>MTDRDRLRPPLDERSLRDQLIGAGSGWRQLDVVAQTGSTNADLLARAASGADIDGVVLIAEHQTAGRGRHGRGWAATARAQIILSVGVRVVDVPVQAWGWLSLAAGLAVLDSVAPLIAVPPAETGLKWPNDVLARGGKLAGILAEVAQPFVVLGVGLNVTQAPEEVDPDATSLLDLGVAAPDRNRIASRLLRELEARIIQWRNANPQLAADYRARSLTIGSRVRVELPGGQDVVGIARDIDDQGRLCLDVGGRTVVVSAGDVVHLR[2x]

Acetyl Coenzyme A Carboxylase (ACC), an important enzyme that catalyzes the first reaction of fatty acid biosynthesis, is biotinylated by biotin acetyl-CoA carboxylase ligase (BirA). The Mtb-BirA molecule is composed of two domains; N-terminal domain 1 comprises of 7 β-strands (β1: 29–32, β2: 55–59, β3: 82–88, β4: 124–126, β5: 131–133, β6: 137–147 and β7: 150–158) and 6 α-helices (α1: 13–20, α2: 39–48, α3: 95–114, α4: 173–176, α5: 183–203, α6: 206–215), while C-terminal domain 2 is a SH3 domain with 5 strands forming an antiparallel β-sheet (β8: 220–227, β9: 231–240, β10: 246–250, β11: 253–257 and β12: 261–264). The two domains are linked together with loop L10 (216–219) that connects helix α6 of domain 1 and β8 strand of domain 2. All the apo BirA crystal structures have revealed the presence of disordered flexible loops, which undergo a conformational transition upon biotin and biotinyl-5′-AMP binding.

Structures of dehydrated (dhMtb-BirA) and hydrated (hMtb-BirA) Mtb-BirA, were determined at 2.69 Å and 2.8 Å, respectively, using crystals grown under similar conditions. The transfer of Mtb-BirA crystals to paraffin and paratone-N oil (cryoprotectants) and subsequent flash freezing resulted in the dehydration of the crystals and significantly reduced their solvent content. The asymmetric unit of dehydrated crystal form containing two molecules is more compact and densely packed with a low solvent content of 28% compared to the hydrated crystal forms. Additionally, the most interesting feature is the appearance of two missing loop regions L4 and L8 and 5 N-terminal residues in subunit A of the dhMtb-BirA. The electron density for loop L8 leaves little doubt as to the position of the atoms and though electron density for loop L4 is not complete, apex of this loop constituting residues R69 and H70 has a well-defined density. The two subunits of dhMtb-BirA have structural differences in their loops and defy the expected two fold symmetry resulting in an asymmetric dimer where, subunit A can be considered a representation of the active ligand bound conformation of BirA and subunit B is more an icon of apo BirA with disordered loops. The maximum deviation of ∼14 Å appears to be in L8 loop, which is adenosine binding loop and may correspond to the conformational shift this loop undergoes upon biotin or biotinyl-5′-AMP binding. Large shift of ∼3.5 Å in the flexible loop L6 as well as in the β8-L11-β9 region is an apparent consequence of crystal dehydration. The ordered loops L4 and L8 in the structure of dehydrated apo BirA form an open, large and spacious biotin-binding pocket. The overall changes in the subunit A of dhMtb-BirA structure appear to mimic those that arise during substrate binding and corroborate well with the established relationship between hydration, mobility and enzyme action.>[10x]MIIMVLQDIDGIFDSQAILAGRFHNDLTVINEKYDLFYLMLPTINEKKIVSFYIFLQDDQIPERHREEIESVLNKFNPVIKNGIWKIYLDTESFKLSEPFSTFFGIDSIVFDMGSMKGGEMLLPVRFISKDKDALVNSIIDSAGYGENIYLRYIGQNKGFDYSFIAIKLLDQVYKLTLSIDNPHVMHGIFAETKKNIAWRRESKAPHKDNTED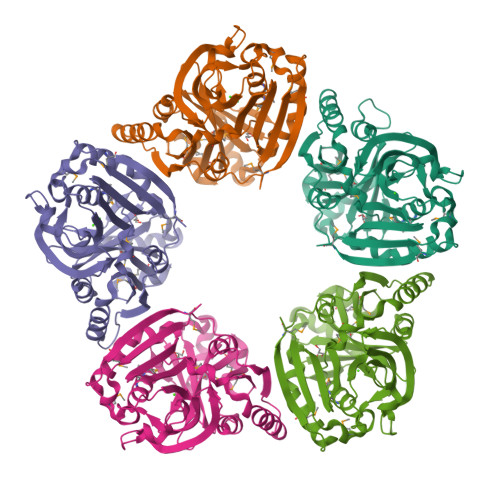YIYALDDTHTIPDILIDTAYTGEKGTVYIGKHSNYDIYRAFFGDALTNHMSSVMISENVYYLRRWSKYEDGKLFLYFYTTVDFLRLIPAILDSTRKNFPKVNMKIDEITPMALEHHHHHH(1-methyl-1H-1,2,3-triazol-4-yl)methyl alpha-D-mannopyranoside | C10 H17 N3 O6 | 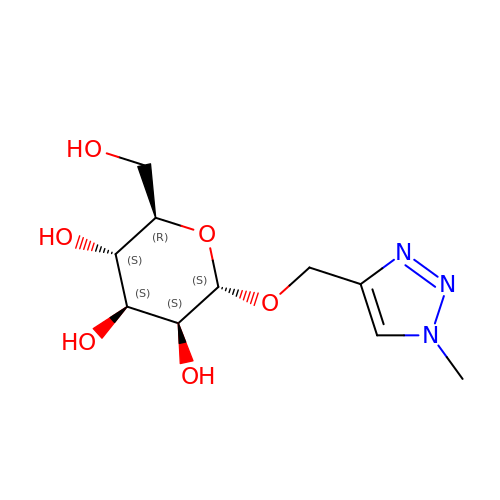GTGCGDYGALMCDQ-ZJDVBMNYSA-N> DYDICKSWVTTDEGPTWEFYACQPKVMRLKDYVKVKVEPS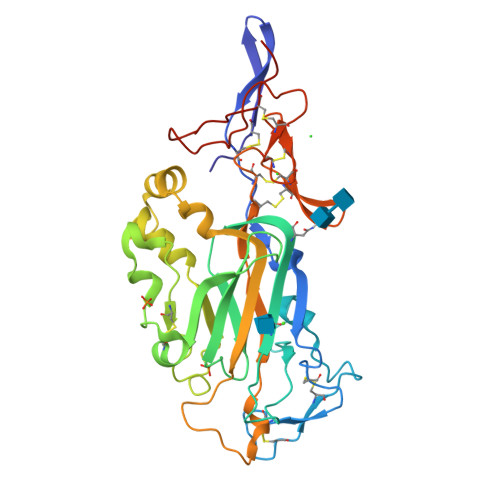GITCGDPPERFCSHENPYLCSNECDASNPDLAHPPRLMFDKEEEGLATYWQSITWSRYPSPLEANITLSWNKTVELTDDVVMTFEYGRPTVMVLEKSLDNGRTWQPYQFYAEDCMEAFGMSARRARDMSSSSAHRVLCTEEYSRWAGSKKEKHVRFEVRDRFAIFAGPDLRNMDNLYTRLESAKGLKEFFTLTDLRMRLLRPALGGTYVQRENLYKYFYAISNIEVIGRCKCNLHANLCSMREGSLQCECEHNTTGPDCGKCKKNFRTRSWRAGSYLPLPHGSPNACAAAGSHHHHHH> GSSRAMGNEVAGVEDISVEITPSSKRNSDARRTSRNVCSNEERKRRKYFHMLYLVCLMVHGFIRNEWINSKRLSRKLSNLVPEKVFELLHPQKDEELPLRSTRKLLDGLKKCMELWQKHWKITKKYDNEGLYMRTWKEIEMSANNKRKFKTLKRSDFLRAVSKGHGDPDISVQGFVAMLRACNVNARLIMSCQPPDFTNMKIDTSLNGNNAYKDMVKYPIFWCEVWDKFSKKWITVDPVNLKTIEQVRLHSKLAPKGVACCERNMLRYVIAYDRKYGCRDVTRRYAQWM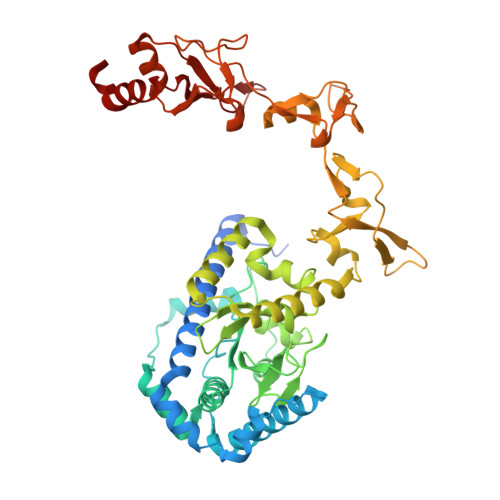NSKVRKRRITKDDFGEKWFRKVITALHHRKRTKIDDYEDQYFFRRDESEGIPDSVQDLKNHPYYVLEQDIKQTQIVKPGCKECGYLKVHGKVGKVLKVYAKRDIADLKSARQWYMNGRILKTGSRCKKVIKRTVGRPKGEAEEEDERLYSFEDTELYIPPLASASGEITKNTFGNIEVFAPTMIPGNCCLVENPVAIKAARFLGVEFAPAVTSFKFERGSTVKPVLSGIVVAKWLREAIETAIDGIEFI>[4x]MGSSHHHHHHSSGENLYFQGHMASGSEFELMGKLDKASKLIDEENKYYARSARINYYNLVIDHAHGATLVDVDGNKYIDLLASASAINV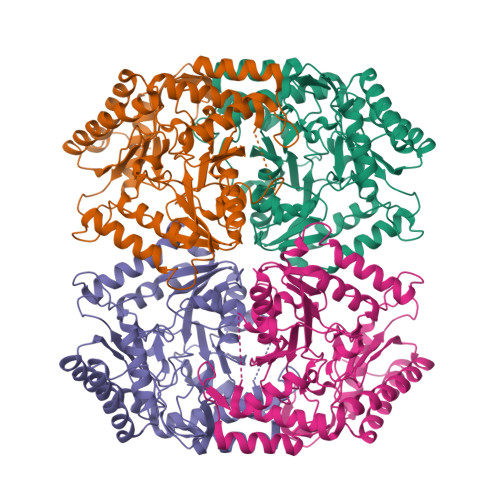GHTHEKVVKAIADQAQKLIHYTPAYFHHVPGMELSEKLAKIAPGNSPKMVSFGNSGSDANDAIIKFARAYTGRQYIVSYMGSYHGSTYGSQTLSGSSLNMTRKIGPMLPSVVHVPYPDSYRTYPGETEHDVSLRYFNEFKKPFESFLPADETACVLIEPIQGDGGIIKAPEEYMQLVYKFCHEHGILFAIDEVNQGLGRTGKMWAIQQFKDIEPDLMSVGKSLASGMPLSAVIGKKEVMQSLDAPAHLFTTAGNPVCSAASLATLDVIEYEGLVEKSATDGAYAKQRFLEMQQRHPMIGDVRMWGLNGGIELVKDPKTKEPDSDAATKVIYYAFAHGVVIITLAGNILRFQPPLVIPREQLDQALQVLDDAFTAVENGEVTIPKDTGKIGW> NLVTPKRELEQGVAFSDLCNFLVTPTVQGWKVYWAGLEFDVNQKGITLLNRLKVNDFAPAWAMTRNLFPHLFKNQQSEVQTPIWALRVILAAGILDQLMDHSLIEPLSGALNLIADWLLTTSTNHFNMRTQRVKDQLSMRMLSLIRSNIINFINKLETLHVVNYKGLLSSVEIGTPSYAIIITRTNMGYLVEVQEPDK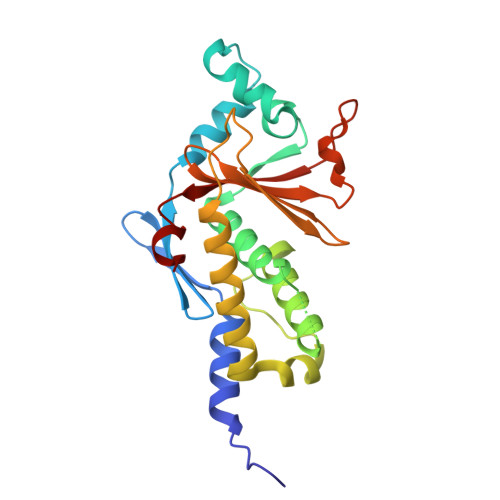SAMDIRHPGPVKFSLLHESTLKPVAT>VKLAAGMGVMSDLEKKFIELEAKLVAQPAGQAMPGKSNIFANNEAWRQEMLKQDPEFFNRLANGQSPEYLWIGCADSRVPANQLLDLPAGEVFVHRNIANQCIHSDISFLSVLQYAVQYLKVKHILVCGHYGCGGAKAALGDSRLGLIDNWLRHIRDVRRMNAKYLDKCKDGDEELNRLIELNVLEQVHNVCATSIVQDAWDAGQELTVQGVVYGVGDGKLRDLGVVVNSSDDISKFYRTKSDSGALKAGNPNAPLVQVTKGGESELDSTMEKLTAELVQQTPGKLKEGANRVFVNNENWRQKMLKQDPQFFSNLAHTQTPEILWIGCADSRVPANQIINLPAGEVFVHRNIANQCIHSDMSFLSVLQYAVQYLKVKRVVVCGHYACGGCAAALGDSRLGLIDNWLRHIRDVRRHNQAEL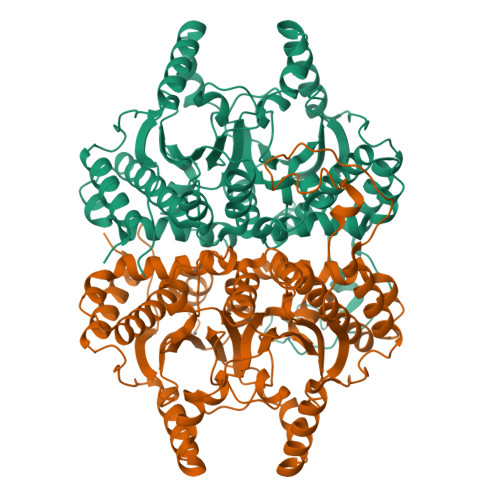SRITDPKDSLNRLIEINVLEQMHNVCATSIVQDAWDAGQELEVQGVVYGVGDGKLRDMGVVAKANDDIGQIFRTKQ[2x]N-(2-{(4-bromophenyl)[(1-methyl-1H-imidazol-5-yl)methyl]amino}ethyl)-1-methyl-N-(2-methylbenzyl)-1H-imidazole-4-sulfonamide 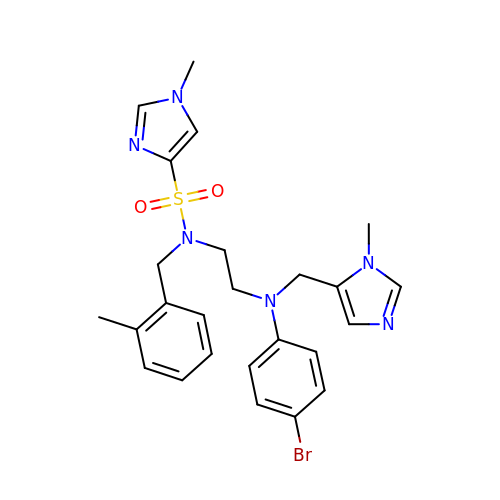| C25 H29 Br N6 O2 S | FOPZJCZMMFSDOL-UHFFFAOYSA-N>HHHHHHSSGLVPRGSMTKIAEKSKQEYGDLLKEKDHLQDMEQLEMTIVSIQTPYPSIVRIQGKINTLQPELWQAP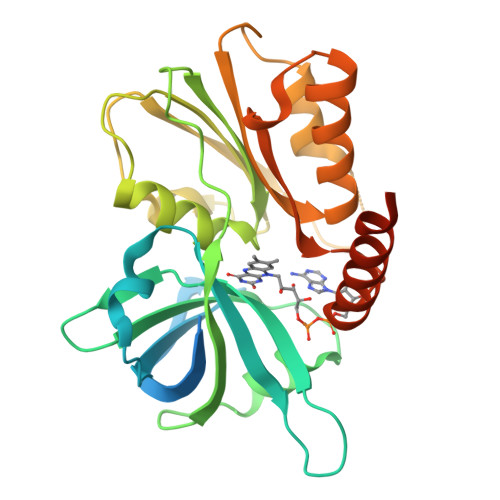NLAIRLIVSNPPEGQPISRVYTVRSFNPINAQIEIDFVKHEDLSPAMEWLNSAQVGTKIGLIGPRPHFIPNFTAKKHVVMFADDTAVPALYSILKQWELGISADIFIESFEKDIASQLPELEHVKIHSFHKEHHTSQKGLLLKAAFALEHYENITIWAACERNEARALRQFFLEDQQLNKNDVRIAGYWRDGVSSSELDKLRAQHYQEHIQQGKTLNEYDDLDLAN[2x]> MNQNLLVTKRDGSTERINLDKIHRVLDWAAEGLHNVSISQVELRSHIQFYDGIKTSDIHETIIKAAADLISRDAPDYQYLAARLAIFHLRKKAYGQFEPPALYDHVVKMVEMGKYDNHLLEDYTEEEFKQMDTFIDHDRDMTFSYAAVKQLEGKYLVQNRVTGEIYESAQFLYILVAACLFSNYPRETRLQ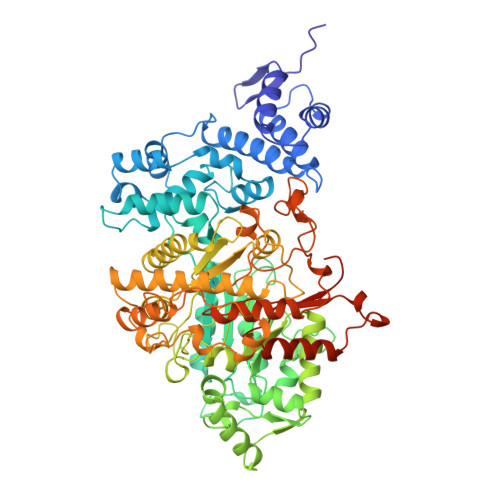YVKRFYDAVSTFKISLPTPIMSGVRTPTRQFSSCVLIECGDSLDSINATSSAIVKYVSQRAGIGINAGRIRALGSPIRGGEAFHTGCIPFYKHFQTAVKSCSQGGVRGGAATLFYPMWHLEVESLLVLKNNRGVEGNRVRHMDYGVQINKLMYTRLLKGEDITLFSPSDVPGLYDAFFADQEEFERLYTKYEKDDSIRKQRVKAVELFSLMMQERASTGRIYIQNVDHCNTHSPFDPAIAPVRQSNLCLDIALPTKPLNDVNDENGEIALCTLSAFNLGAINNLDELEELAILAVRALDALLDYQDYPIPAAKRGAMGRRTLGIGVINFAYYLAKHGKRYSDGSANNLTHKTFEAIQYYLLKASNELAKEQGACPWFNETTYAKGILPIDTYKKDLDTIANEPLHYDWEALRESIKTHGLRNSTLSALMPSETSSQISNATNGIEPPRGYVSIKASKDGILRQVVPDYEHLHDAYELLWEMPGNDGYLQLVGIMQKFIDQSISANTNYDPSRFPSGKVPMQQLLKDLLTAYKFGVKTLYYQNTRDGAEDAQDDLVPSIQDDGCESGACKI>[2x]MHHHHHHSSGSMQIEIKDGRSDNSPLPERKLVTLIQESYDSLKDDNEINLSTESTSNLLIKLVLEKLEKHSSLYKYIA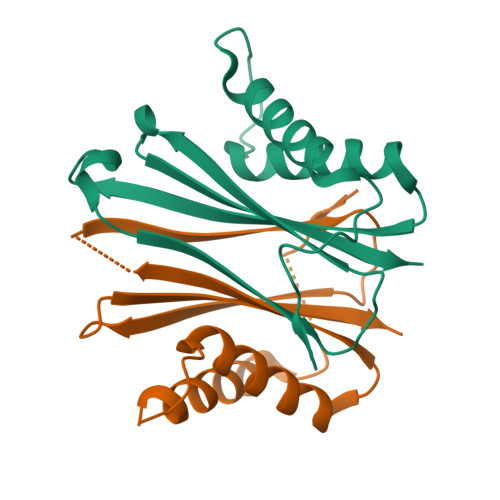SVTTLNIEGLNEENANFSLKNDIGASWESKKDGIFNYKLEDKNNNECYLITILWLHK>[4x]GSDKRGPQSAEPDPLERLEVKKVQQQHENEKDDSGRDTKSGGKVAKAMTKGDTIAGKLLTTPSRLFKLLIPLTT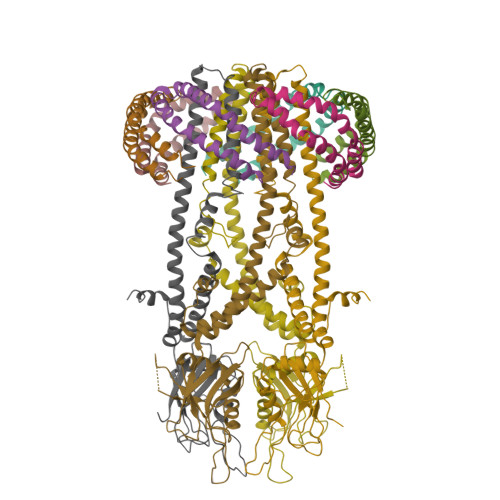INRKDIEQIAILIHPQQPLSHLERLIQSEVPPIEDENGQKRPPFVSFIALQLEQDAIRPKRGMYEGTDAEIHRVEGGKDDATVAKRGEDFQEVDETFSYLRRPGPGQGDKEQRFIRWSQSTEIGDFIRDAARAKEFIVTIEGAPAGLEQIHVAVPSFDERTYFLRMRLRKISRRIQGLAEIKHECDALAHRGAQRVALGGFGILAFWWYIVYKLTFETDLGWDTMEPVTYLVSLSTLMGGYLWFLYHNREISYRSALDFTINARQKKLYQMKGIDLQVWESLIDEANAIRREIKNIAAEYDVDWDERKDEQDDRVTEALKKERRLKNGSQKEERPKDDRDDD N-{4-[(4S,10aP)-8-chloro-2-methyl-5-oxo-5,6-dihydro[1,2,4]triazolo[1,5-c]quinazolin-9-yl]-3-methylphenyl}methanesulfonamide 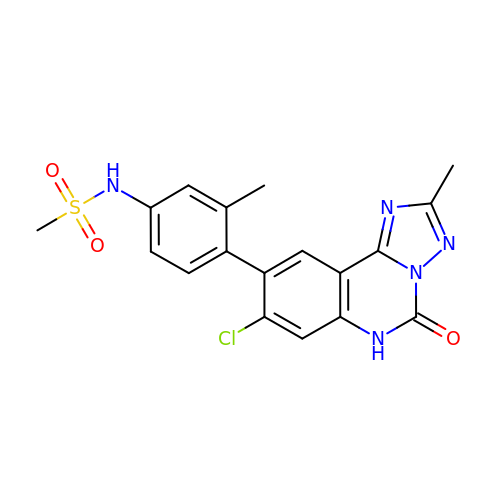| C18 H16 Cl N5 O3 S | RXWRFWXLZLLXSL-UHFFFAOYSA-N>[2x]MSEDIRRGPGRPPKKRVVPNFERKGILEKPVRPQSRLEFSYDNPLIFKNLFIYFKNLKSKNILVRCTPTEITFFSRDQSQASFVIATIDGKNVNHYYASDVFWLGINRELVEKMFNSIDRSFLKITI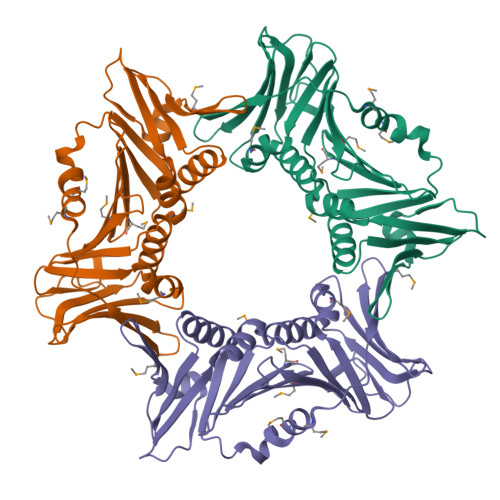VHRYDKPETLFFIFTDFDIDKECTYQITVSEPELDMDLIEMEKSISEERLKNYPLRWEFTSKQLKKTFSDLSNYTELVTIEKLGGDTPLHLYFQKFNSISYHEMYKSSNKINLTSTIPKSQVFQINVKIAHIKSLASAMVTDKIRILCEENGNLIFQSEMDALMLNTITLNNTIGSSSHHHHHH> MHHHHHHSMGKRNKPGKATGKGKPVNNKWLNNAGKDLGSPVPDRIANKLRDKEFKSFDDFR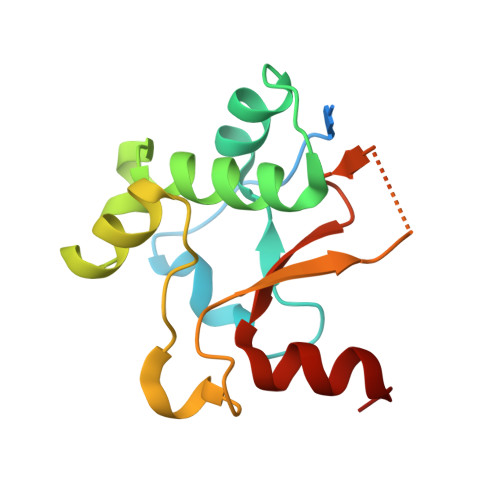KKFWEEVSKDPELSKQFSRNNNDRMKVGKAPKTRTQDVSGKRTSFELHAEKPISQNGGVYDMDNISVVTPKRHIDIHRGK>MGLTPLMIAAVRGGGLDTGEDIENNEDSTAQVISDLLAQGAELNATMDKTGETSLHLAARFARADAAKRLLDAGADANSQDNTGRTPLHAAVAADAMGVFQILLRNRATNLNARMHDGTTPLILAARLAIEGMVEDLITADADINA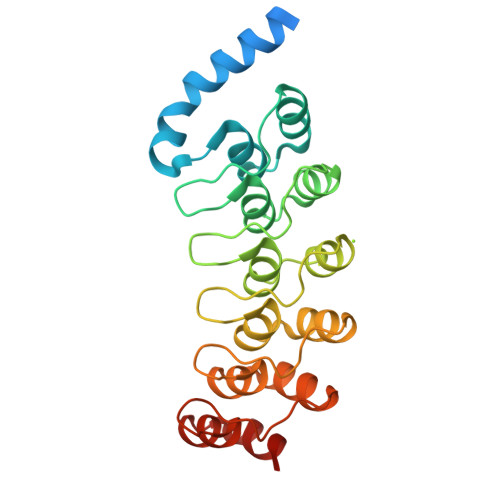ADNSGKTALHWAAAVNNTEAVNILLMHHANRDAQDDKDETPLFLAAREGSYEASKALLDNFANREITDHMDRLPRDVASERLHHDIVRLLDEH[3x]α-Actinin-2 (ACTN2) is the only muscle isoform of α-actinin expressed in cardiac muscle. All four isoforms of α-actinin consist of an N-terminal actin binding domain (ABD) comprising two calponin homology (CH) domains, connected via a flexible linker, which allows for conformational flexibility in the ABDs, to a rod domain. Thus ACTN2 is important in cross-linking actin and titin filaments in the Z-disc. We have investigated the effects of two mutations identified from HCM patients, A119T and G111V, on the secondary and tertiary structure of a purified actin binding domain (ABD) of ACTN2 by circular dichroism and X-ray crystallography, and show small but distinct changes for both mutations.

To determine how these two mutations might contribute to HCM, we have expressed and purified the ABD comprising the two CH domains from human ACTN2, together with two mutant variants A119T (AT) and G111V (GV) and determined their structure, and actin binding affinity. We were successful in obtaining crystals for the WT and both mutant ABDs and were able to solve their structures to a resolution of between 1.9 and 2.2 Å. The ABD was in the ‘closed’ conformation in all the structures, as found for other structures of the ABDs for the second striated muscle isoform ACTN3, and the two non-muscle isoforms ACTN1. In the closed conformation that we observed, there is extensive contact between the CH1 and CH2 domains, and the residues Arg243 and Trp145 stack together, as found for other ACTN ABDs. Intriguingly, one of our two structures for the WT construct contains an additional N-terminal α-helix, upstream of the first CH1 domain not seen previously. From our structures of the other WT and the two mutants that do not have this N-terminus helix, this may suggest that the N-terminus is highly flexible. For both the WT and A119T mutant structure, Val112 is orientated towards the interior of the molecule packing the side chain into a hydrophobic region. The measured Kd for the WT construct of 7.5 μM, is comparable to that measured for other ACTN ABDs [∼1 μM for smooth muscle ACTN (ACTN1), and 5 μM for Acanthamoeba ACTN]. Thermal denaturation experiments showed that the thermal stability for both mutants was lower than that for the WT construct.

>GPYMIQEEEWDRDLLLDPAWEKQQRKTFTAWCNSHLRKAGTQIENIEEDFRNGLKLMLLLEVISGERLPKPDRGKMRFHKIANVNKALDYIASKGVKLVSIGAEEIVDGNVKMTLGMIWTIILRFAIQDISVEETSAKEGLLLWCQRKTAPYRNVNIQNFHTSWKDGLGLCALIHRHRPDLIDYSKLNKDDPIGNINLAMEIAEKHLDIPKMLDAEDIVNTPKPDERAIMTYVSCFYHAFAGAEQAETAA[2x]>MVRPSQSMYDRHLTIFSPDGNLYQIEYAIKAVKNTNITSVGVKGENCAVIISQKKMATQYISQDKLLDYNNITNIYNITDEIGCSMVGMPGDCLSMVYKARSEASEFLYSNGYNVNAETLCRNICDKIQVYTQHAYMRLHACSGMIIGIDENNKPELFKFDPSGFCAGYRACVIGNKEQESISVLERLLEKRKKKIQQETIDEDIRNTTILAIEALQTILAFDLKASEIEVAIVSTKNRNFTQISEKEIDNYLTYIAERD[2x];>[2x]MADGEYSFSLTTFSPTGKLVQIEYALNRVSSSSPALGIRAKNGVIIATEKKSPNELIEENSIFKIQQISEHIGIVYAGMPGDFRVLLKRARKEAIRYSLQYGSEILVKELVKIIASIVQEFTQTGGVRPFGLSLLICGVDVYGYHLYQIDPSGCYFNWMATCVGKDYQNNMSFLEKRYNKDIEIEDAIHTAILTLKESYEGVLNEKNIEIGVAYDNKPFKILTQNEIKDYLIEIE;>[2x]MARRYDSRTTTFSPEGRLYQVEYALEAINNASITIGLITKDGVILGADKVFISKLIDKANNYEKIYKIDKHIFCGVAGLNADANILINQSRLYAQRYLYNYNEVQPVSQLVVQICDIKQSYTQYGGLRPYGVSFLIGGYDTKDGYQLYHTDPSGNYSGWFATAIGTNNLTASSVLKQEWKNDMTLEEGLLLALKTLAKSTDTEIPKSEKIELAYLTNKDGEVYQKYLTEKEIEELIKLYTQKYIKE;>[2x]MSYDRAITVFSPDGHLLQVEHALEAVKKGGCAVAIKSSNFAVLAVEKKNIPKLQNPKTTEKLIKLDEHNCLAFAGLNADARVLVNKTRLECQRYYLNMDEPAPVDYIAKYVAKVQQKFTHRGGVRPFGIATLIAGFKNNKEICIYQTEPSGIYAAWKAQAIGKNAKIVQEFLEKNYQENMEQKDCIFLALKAIFEVVELSSKNVEVALLTEKDLTFIEEQEINSMVELIDQERTKNNEQNE;>[2x]MFSTRSEYDRGVNTFSPEGRLFQVEYALGAIKLGSTAVGICVNDGVILASERRISSTLIEKDSVEKLLSIDDHIGCAMSGLMADARTLIDYARVECNHYKFIYNENINIKSCVELISELALDFSNLSDSKRKKIMSRPFGVALLIGGVDKNGPCLWYTEPSGTNTRFSAASIGSAQEGAELLLQENYKKDMTFEQAEILALTVLRQVMEDKLSTSNVEICAIKKSDQTFYKYNTDDISRIIDVLPSPVYPTIDMTA;>MYRNLYDTDNIIYSPEGRLYQVEYASEAIKQGTCAVAIKSKDYVVVSGLKKCISKLSFPQEKIFKIDDYIGISMSGITSDAKVLTKFMQNECLSHKFLYNENINIESLVRSVADKYQKNTQKSSKRAFGVGLMIAAYHNEPCIFETRPNGSYFEYDALSFGARSHASKTYLEKNLHLFEECSLEELILHCLKALKCSLSS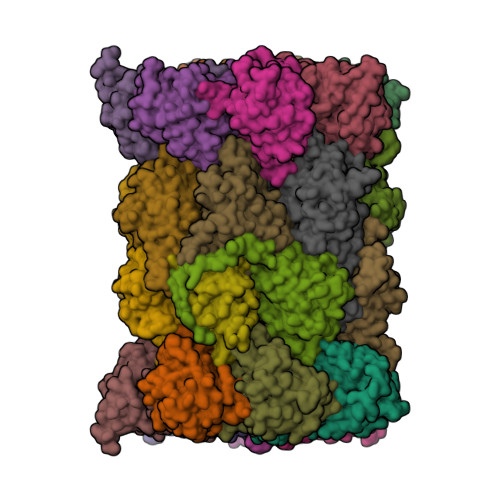ESELTISNTALAVVGKNHPWQEISSLQLEEYLSKVKMDAEQEQVEENVQNEAN[2x];>[2x]MAGLSAGYDLSVSTFSPDGRLYQVEYIYKSINNNNTALCLECKDGIICCCINSNMDKNKMIKKNSYNRIYHVNNNIIITYSGFDGDARNIIDRARSEANTYYYNFHTNIPLHILVNRISLYIHAYTLYWHMRPFAASIIISSFNEKDKGDIYCIEPNGACYKYSGIVIGKNKEMFKTEIEKKDYKDINVRDAIEDIYKFILTSDDHMNKNNLQNLVNFSWICKESSYEFQNIHEEILTPALNKAVEYIEKLN;>TTIIGIIYDNGVMLACDSRTSSGTFISNKCSRKINRINENLYVCRSGASAHSQKIIEIIKHYCVSMKNENRKKGRFHEGETIYDETTYDEEIDIDSINYLDYNNNNDNNLVTKNKYFYEDKFNDYNPLVENVAHITKKIIYTNNNFLSCALIFGGYDKIKKQQLYAVNLNGSIIEKHDFAVSGSGSIYIQSYLQDKYKKFMTKKECFNLILNCVKYAMHNDNSSGGLIRIVNITKSFVEEFTVVNTQMNFQY[2x];>TTICGLVCQNAVILGADTRATEGPIVADKNCSKLHYISKNIWCAGAGVAGDLEHTTLWLQHNVELHRLNTNTQPRVSMCVSRLTQELFKYQGYKVCAIVLGGVDVNGPQLYGIHPHGSSCLLPFTALGSGSLNAMAVLEAKYRDNMTIEEGKNLVCEAICAGIFNDLGSGGNVDICVITKDSYQHIRPYKEPNMRLYHLPHPTIYPKGTTPILSEKIEYIKKFISVEDA[2x];>MGSIYNYNGGCVLGMSGSNCVAIACDLRLGANTFTTVSTKFSKIFKMNNNVYVGLSGLATDIQTLYEILRYRVNLYEVRQDAEMDVECFANMLSSILYSNRFSPYFVNPIVVGFKLKHYVDEEGEKKVNYEPYLTAYDLIGAKCETRDFVVNGVTSEQLFGMCESLYVKDQDENGLFETISQCLLSALDRDCISGWGAEVLVLTPEKIIKKKLKARMD[2x];>MDTLIGLRGNNFVVLAADTYSINSIIKLKNDDNTKFYDIHGNKCLLLGGSIGDRLQFGEFIRKNVHLYQYQNNTDMFVKSFAFFTRKNLAYYLRRNPFEVNCLIAGYDKKDGYQLYWCDYLSNMDSVNKGAHGYGAYLVSAILDKYYHENLTVDEALDIFKLCFEELKKRFLLTQINYELRIMYDNKVETQYVTV[2x];>[2x]TTTLAFKFKDGIIVAVDSRASMGSFISSQNVEKIIEINKNILGTMAGGAADCLYWEKYLGKIIKIYELRNNEKISVRAASTILSNILYQYKGYGLCCGIILSGYDHTGFNMFYVDDSGKKVEGNLFSCGSGSTYAYSILDSAYDYNLNLDQAVELARNAIYHATFRDGGSGGKVRVFHIHKNGYDKIIEGEDVFDLHYHYTNPEQKDQYVM;>MDLILYNDNLTEKKTEKENVIEHGRGFKRWYPYIDNGGTVIGLTGKDYVILAADTRLSLSYSIYTRFCPKISKLTDKCIIGSSGMQSDIKTLHSLLQKKIQLFVLEHSHYPDIHVIARLLCVILYSRRFFPYYAFNILAGVDENNKGVLYNYDSVGSYCEATHSCVGSGSQLILPILDNRVEQKNQLIKNTNFNLGDDINFVKDAITSATERDIYTGDKTLIYVIDKMGINVNTLDLKQD[2x];>MTLGPVVTGTSVIAIKYKHGIMIAADRKASYGSYAKFQNVERIFKINNKTVMGFSGELADAQYLHELLTRKNINNLSEKKRKEDMYTPQHYHSYVSRVFYVRKNRIDPLFNNIIIAGINSQKYDNNDDNVLLYTNKNNDDEQNEYKNNEEYKEIHKDDLYIGFVDMHGTNFCDDYITTGYARYFALTLLRDHYKDNMTEEEARILINECLRILYFRDATSSNFIQIVKVTSKGVEYEEPYILPCVLNSADYVYPSTLLPPAGCMW[2x]>MSDTLPGTTLPDDNHDRPWWGLPCTVTPCFGARL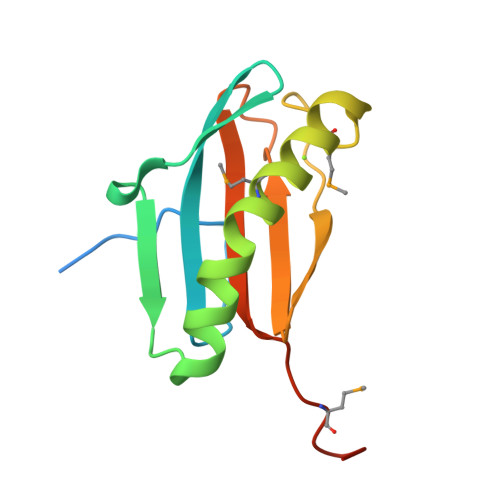VQEGNRLHYLADRAGIRGLFSDADAYHLDQAFPLLMKQLELMLTSGELNPRHQHTVTLYAKGLTCKADTLSSCDYVYLAVYPTPEMKNLEHHHHHH[2x]>[2x]SVQPNFQQDKFLGRWFSAGLASNSSWLREKKAALSMAKSVVAPATDGGLNLTSTF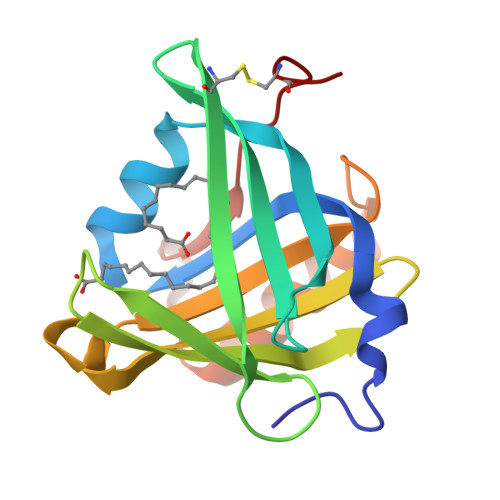LRKNQCETRTMLLQPAGSLGSYSYRSPHWGSTYSVSVVETDYDQYALLYSQGSKGPGEDFRMATLYSRTQTPRAELKEKFTAFCKAQGFTEDTIVFLPQTDKCMTEQ>MGSSHHHHHHSGLVPRGSHMATPPKRSSPSFSASSEGTRIKKISIEGNIAAGKSTFVNILKQLSEDWEVVPEPVARWSNVQSTQDEFEELTMSQKNGGNVLQMMYEKPERWSFTFQTYACLSRIRAQLASLNGKLKDAEKPVLFFER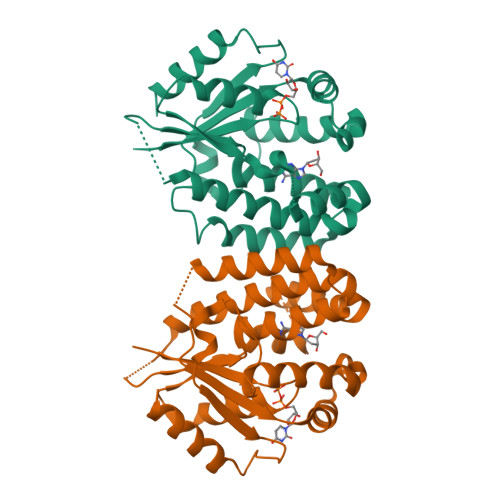SVYSDRYIFASNLYESESMNETEWTIYQDWHDWMNNQFGQSLELDGIIYLQATPETCLHRIYLRGRNEEQGIPLEYLEKLHYKHESWLLHRTLKTNFDYLQEVPILTLDVNEDFKDKYESLVEKVKEFLSTL[4x]>[12x]MGSSHHHHHHSSGLVPAGSHSKVFIRSAINRVHQNSAANGGELPRIVFPEGTSTKV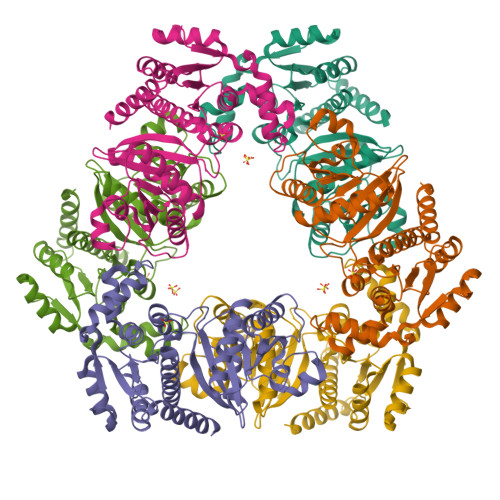LKALATLVEEKICQPILLGYPERVKEKIKALDIPLLNDVSIVHPSSHPKYFSFVEKLYSLRQRKGINLGEAERLMADPNYFAAMMVNQGEADGMVSGSSINYADAVRPILQTIGVYKEGIPAGLNFVLLEDKFLVLADTTVNLNPTAEQCAQIALQAAKIVEYFGIEPRVAMLSYSNFSGAEGTPRKMKKAAEIARSLRPDLMIEGDMQADTAVNPEIMERLFPFSGLKGGANVLVFPNLESSDIAYKLIQQIGKAEVIGPFLTGVRRSANVLQRTTTVDGIVNSVVFTALEAQYIKEVLKSRGKK> MSEKTVLSIQSFVTHGYVGNKAATFPLQLHGFDVDGINTVCLSNHSGYPVIRGHRMSLQEYDELMEGVRANNFLSNYRYILTGYINNVDIIGRIRDTLKEVRELREKEDKKLTFICDPVMGDDGIMYCKKEVLDAYRELVPLADIVTPNYFEASLLSGVTVNDLSSAILAADWFHNCGVAHVIIKSFREQENPTHLRFLYSVKEGSEAAVRRFSGVVPYHEGRYTGTGDVFAACLLAFSHSHPMDVAIGKS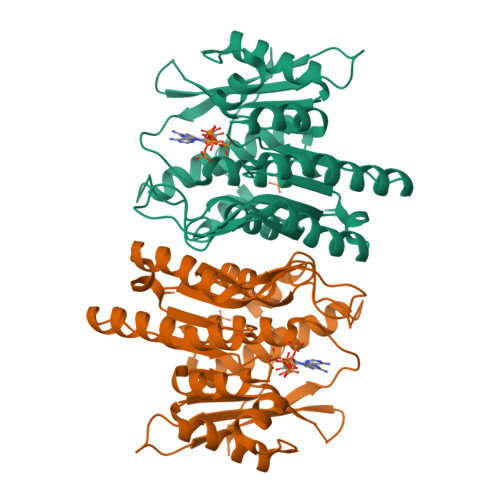MAVLQELIIATRKEGGDGKSSLKSRELRVVASPQVVLQPSTVVDVKPIS> GGDDATASQRGIVTQVADTVSS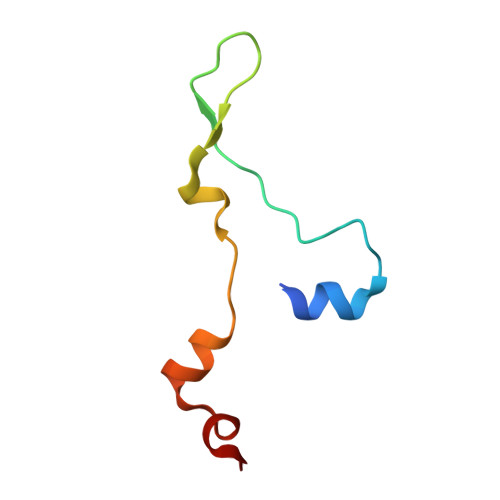ISNVVDGLGVPLLSSISKPIGWVSNVVSNVASIFGF>[4x]MAGGRVRNIGDVMEHPLVELGVSYAALLSVIVVVVEYTMQLSGEYLVRLYLVDLILVIILWADYAYRAYKSGDPAGYVKKTLYEIPALVPAGLLALIEGHLAGLGLFRLVRLLRFLRILLIISRGSKFLSAIADAADKIRFYHLFGAVMLTVLYGAFAIYIVEYPDPNSSIKSVFDALWWAVVTATTVGYGDVVPATPIGKVIGIAVMLTGISA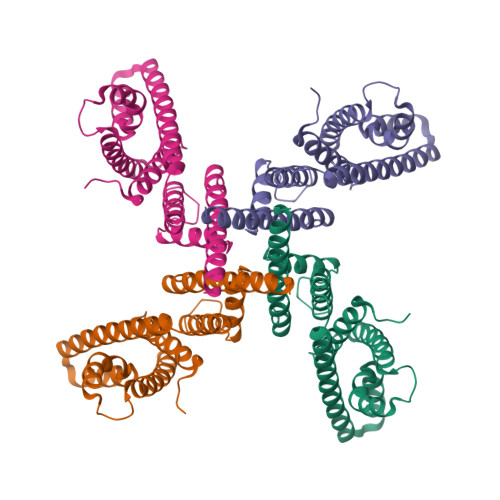LTLLIGTVSNMFQKILVGEPEPSSSPAKLAEMVSSMSEEEFEEFVRTLKNLRRLENSMKLVPRGSRSHHHHHH> GCRYIPSLPDRILDAPEIRNDYYLNLVDWSSGNVLAVALDNSVYLWSASSGDILQLLQMEQPGEYISSVAWIKEGNYLAVGTSSAEVQLWDVQQQKRLRNMTSHSARVGSLSWNSYILSSGSRSGHIHHHDVRVAEHHVATLSGHSQEVCGLRWAPDGRHLASGGNDNLVNVWPSAPGEGGWVPLQTFTQHQGAVKAVAWCPWQSNVLATGGG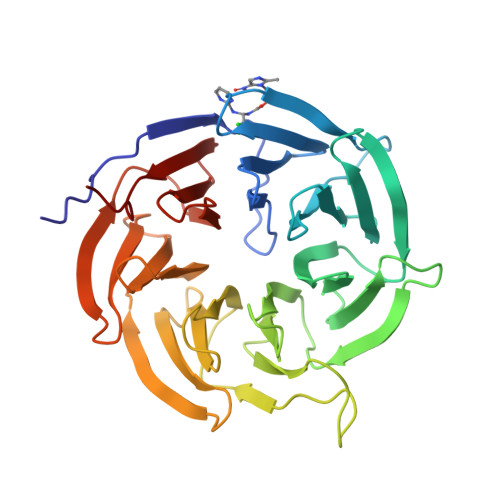TSDRHIRIWNVCSGACLSAVDAHSQVCSILWSPHYKELISGHGFAQNQLVIWKYPTMAKVAELKGHTSRVLSLTMSPDGATVASAAADETLRLWRCFELDP>MQRRDFLKYSVALGVASALPLWSRAVFAAERPTLPIPDLLTTDARNRIQLTIGAGQSTFGGKTATTWGYNGNLLGPAVKLQRGKAVTVDIYNQLTEETTLHWHGLEVPGEVDGGPQGIIPPGGKRSVTLNVDQPAATCWFHPHQHGKTGRQVAMGLAGLVVIEDDEILKLMLPKQWGIDDVPVIVQDKKFSADGQIDYQLDVMTAAVGWFGDTLLTNGAIYPQHAAPRGWLRLRLLNGCNARSLNFATSDNRPLYVIASDGGLLPEPVKVSELPVLMGERFEVLVEVNDNKPFDLVTLPVSQMGIAI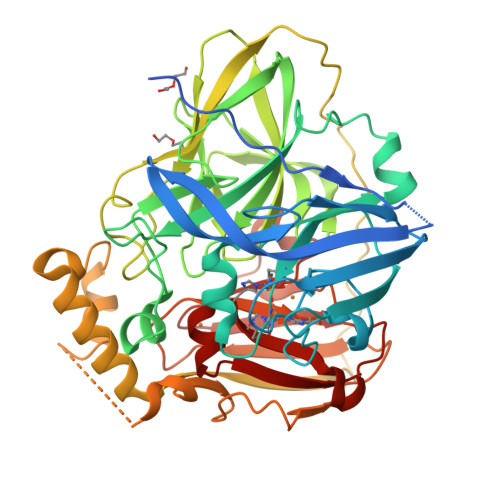APFDKPHPVMRIQPIAISASGALPDTLSSLPALPSLEGLTVRKLQLSMDPMLDMMGMQMLMEKYGDQAMAGMDHSQMMGHMGHGNMNHMNHGGKFDFHHANKINGQAFDMNKPMFAAAKGQYERWVISGVGDMMLHPFHIHGTQFRILSENGKPPAAHRAGWKDTVKVEGNVSEVLVKFNHDAPKEHAYMAHCHLLEHEDTGMMLGFTV[2x]> GTTKH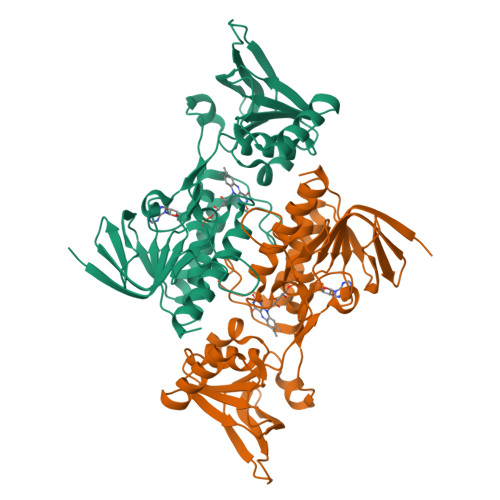SKLLILGSGPAGYTAAVYAARANLQPVLITGMEKGGQLTTTTEVENWPGDPNDLTGPLLMERMHEHATKFETEIIFDHINKVDLQNRPFRLNGDNGEYTCDALIIATGASARYLGLPSEEAFKGRGVSACATSDGFFYRNQKVAVIGGGNTAVEEALYLSNIASEVHLIHRRDGFRAEKILIKRLMDKVENGNIILHTNRTLEEVTGDQMGVTGVRLRDTQNSDNIESLDVAGLFVAIGHSPNTAIFEGQLELENGYIKVQSGIHGNATQTSIPGVFAAGDVMDHIYRQAITSAGTGCMAALDAERYLDGLADAK> KPFTLPVLTIGEMTNSRFPAPIDMLYTSPNGNVVVQPQNGRCTLDGELQGSTQLVPANVCAFRGKITARIVDQAAHQWHMQIDNPNGTLFDPTEDVPA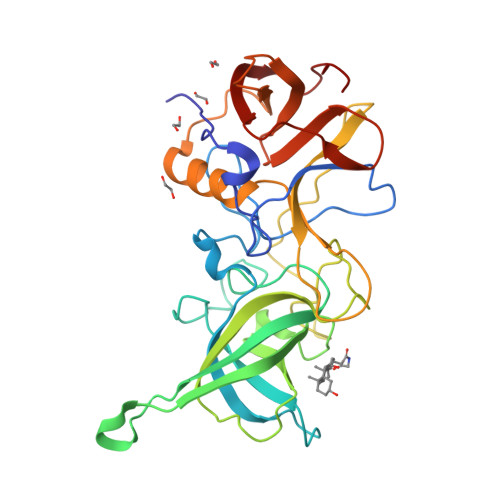PLGTPDFKAKIFGVISQRNDYNDGSQGPANRAHDAVVPTTSAKFTPKLGSILVGTWENNDIETQPSKFTPVGLLEMNDFNQWSLPNYSGALTLNMGLAPAVFPTFPGEQILFFRSFIPLKGGHGNPAIDCLLPQEWIQHFYQESAPSQTSVALIRYVNPDTGRVLFEGKLHRQGFITIAKSGDGPIVVPPNGYFRFDSWVNQFYSLAPM>[5x]PPERGGAGTSQDGTSKNWFKITIPYGRKYDKAWLLSMIQSKCSVPFTPIEFHYENTRAQFFVEDASTASALKAVNYKILDRENRRISIIINSSAPPHTILNELKPEQVEQLKLIMSKRYDGSQQVLDLKGLRSDPDLVAQNIDVVLNRRSCMAATLRIIEENIPELLSLNLSNNRLYRLDDMSSIVQKAPNLKILNLSGNELKSERELDKIKGLKLEEL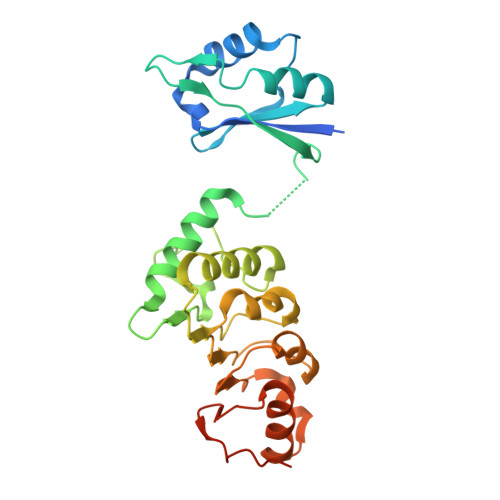WLDGNSLCDTFRDQSTYISAIRERFPKLLRLDGHELPPPIAFDVEAPTTLPP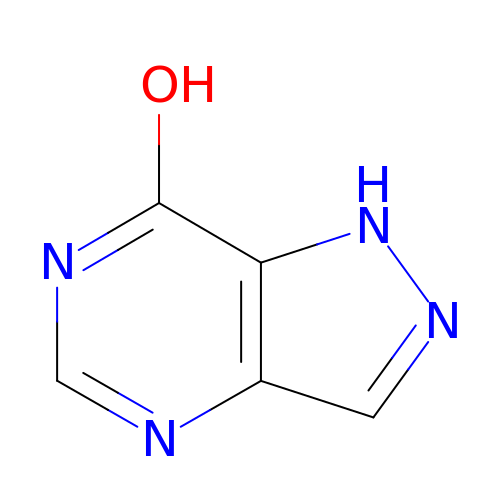7-HYDROXY-PYRAZOLO[4,3-D]PYRIMIDINE | C5 H4 N4 O | JFZSDNLQDTYVEE-UHFFFAOYSA-N>MTHQTHTIAESNNFIVLDKYIKAEPTGDSYQSESDLERELIQDLRNQGYEFISVKSQSAMLANVREQLQNLNGVVFNDSEWRRFTEQYLDNPSDGILDKTRKIHIDYICDFIFDDERLENIYLIDKKNLMRNKVQIIQQFEQAGSHANRYDVTILVNGLPLVQIELKKRGVAIREAFNQIHRYSKESFNSENSLFKYLQLFVISNGTDTRYFANTTKRDKNSFDFTMNWAKSDNTLIKDLKDFTATCFQKHTLLNVLVNYSVFDSSQTLLVMRPYQIAATERILWKIKSSFTAKNWSKPESGGYIWHTTGSGKTLTSFKAARLATELDFIDKVFFVVDRKDLDYQTMKEYQRFSPDSVNGSENTAGLKRNLDKDDNKIIVTTIQKL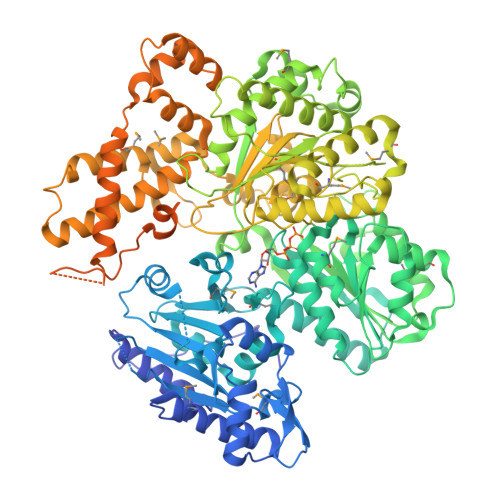NNLMKAESDLPVYNQQVVFIFDECHRSQFGEAQKNLKKKFKRYYQFGFTGTPIFPENALGSETTASVFGRELHSYVITDAIRDEKVLKFKVDYNDVRPQFKSLETETDEKKLSAAENQQAFLHPMRIQEITQYILNNFRQKTHRTFPGSKGFNAMLAVSSVDAAKAYYATFKRLQEEAANKSATYKPLRIATIFSFAANEEQNAIGEISDETFDTSAMDSSAKEFLDAAIREYNSHFKTNFSTDSNGFQNYYRDLAQRVKNQDIDLLIVVGMFLTGFDAPTLNTLFVDKNLRYHGLMQAFSRTNRIYDATKTFGNIVTFRDLERSTIDAITLFGDKNTKNVVLEKSYTEYMEGFTDAATGEAKRGFMTVVSELEQRFPDPTSIESEKEKKDFVKLFGEYLRAENILQNYDEFATLKALQQIDLSDPVAVEKFKAEHYVDDEKFAELQTIRLPADRKIQDYRSAYNDIRDWQRREKEAEKKEKSTTDWDDVVFEVDLLKSQEINLDYILGLIFEHNRQNKGKGEMIEEVKRLIRSSLGNRAKEGLVVDFIQQTNLDDLPDKASIIDAFFTFAQREQQREAEALIKEENLNEDAAKRYIRTSLKREYATENGTELNETLPKLSPLNPQYKTKKQAVFQKIVSFIEKFKGVGGKI[2x]> MREYKLVVVGSGGVGKSALTVQFVQGIFVEKYDPTIEDSYRKQVEVDAQQCMLEILDTAGTEQFTAMRDLYMKNGQGFALVYSITAQSTFNDLQDLREQILRVKDTDDVPMILVGNK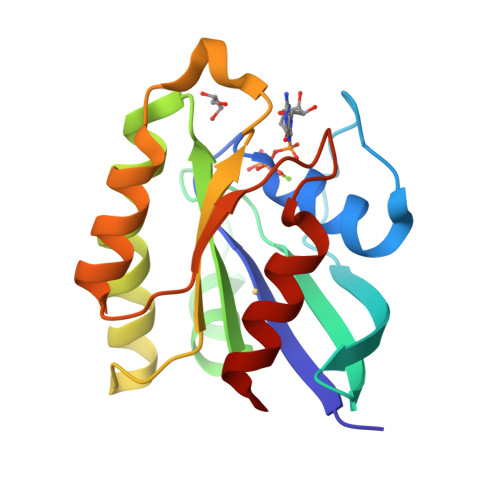CDLEDERVVGKEQGQNLARQWSNCAFLESSAKSKINVNEIFYDLVRQINR>SMASNAARVVATAKDFDKVGLGIIGYYLQLYAVELILSEEDRSQEMTALATELLDTIEAFKKEIGGESEAEDSDKSLHVM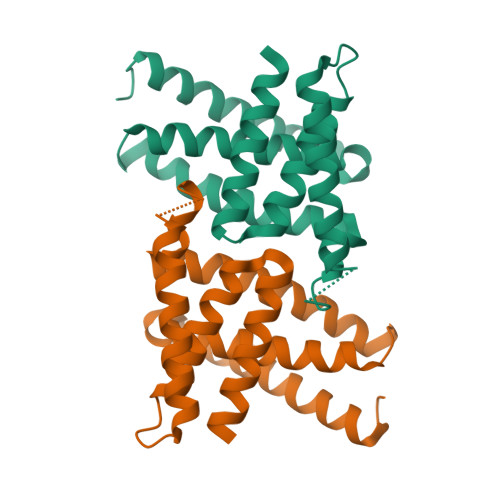NTLIHDQEKAKIYMLNFTMSLYNEKLKQLKDGPWDVMLKRSLWCCIDLFSCILHLWKENISETSTNSLQKRIKYCKIYLSKLAKGEIG[2x]> GPLGMATEEAIIRIPPYHYIHVLDQNSNVSRVEVGPKTYIRQDNERVLFAPVRMVTVPPRHYCIVANPVSRDAQSSVLFDVTGQVRLRHADQEIRLAQDPFPLYPGELLEKDITPLQVVLPNTALHLKALLDFEDKNGDKVMAGDEWLFEGPGTYIPQKEVEVVEIIQATVIKQNQALRLRARKECFDRDGKERVTGEEWLVRSVGAYLPAVFEEVLDLVDAVILTEKTALHLRARQNFKDLRGVAHRTGEEWLVTVQDTEAHVPDVYEEVLGVVPITTLGPRHYC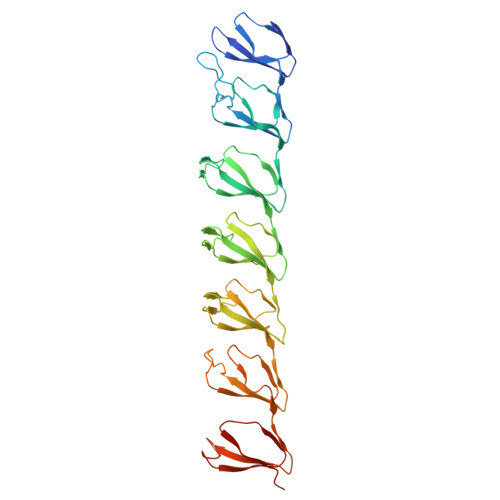VILDPMGPDGKNQLGQKRVVKGEKSFFLQPGERLERGIQDVYVLSEQQGLLLKALQPLEEGEGEERVAHQAGDRWLIRGPLEYVPSAKVEVVEERQAIPLD>GAASRDDEYDYLFKVVLIGDSGVGKSNLLSRFTRNEFNLESKSTIGVEFATRSIQVDGKTIKAQIWDTAGLERYRAITSAYYRGAVGALLVYDIAKHLTYENVERWLKELRDHADSNIVIMLVGNKSDLRHLRAVPTDEARAFAEKNGLSFIETSALDSTNVEAAFQTILTEIYRIVSQKQMSDRRE[8x];>GAASNKSTSSAMSGSHQDLSVIQPIVKDCKEADLSLYNEFRLWKDEPTMDRTCPFLDKIYQEDIFPCLTFSKSELASAVLEAVENNTLSIEPVGLQPIRFVKASAVECGGPKKCALTGQSKSCKHRIKLGDSSNYYYISPFCRYRITSVCNFFTYIRYIQQGLVKQQDVDQMFWEVMQLRKEMSLAKLGYFKEEL[8x];>GAASGAKSLFSTAFSESLAAEISSVSRDELMEAIQKQEEINFRLQDY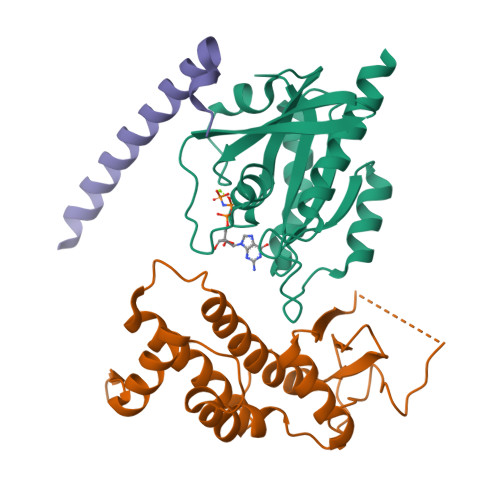IDRIIVAIMETNPSILEVK[8x]>MAIAQLATEYVFSDFLLKEPTEPKFKGLRLELAVDKMVTCIAVGLPLLLISLAFAQEISIGTQISCFSPSSFSWRQAAFVDSYCWAAVQQKNSLQSESGNLPLWLHKFFPYILLLFAILLYLPPLFWRFAAAPHICSDLKFIMEELDKVYNRAIKAAKSARDLDMRDGACSVPGVTENLGQSLWEVSESHFKYPIVEQYLKTKKNSNNLIIKYISCRLLTLIIILLACIYLGYYFSLSSLSDEFVCSIKSGILRNDSTVPDQFQCKLIAVGIFQLLSVINLVVYVLLAPVVVYTLFVPFRQKTDVLKVYEILPTFDVLHFKSEGYNDLSLYNLFLEENISEVKSYKCLKVLENIKSSGQGIDPMLLLTNLGMIKMDVVDGKTPMSAEMREEQGNQTAELQGMNIDSETKANNGEKN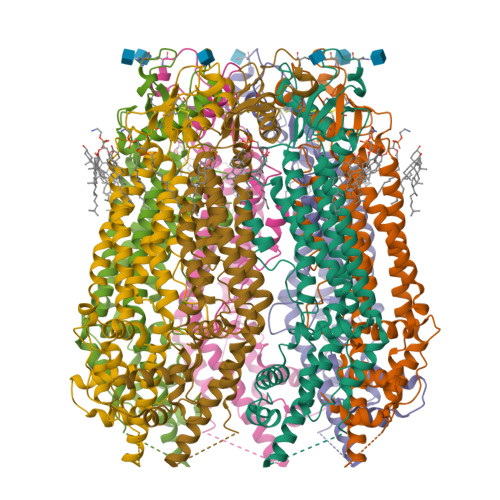ARQRLLDSSC[7x]>[2x]AQPTNFHDQLKFAWLAGFVDADGCINAQIVSREDYLLKYQVRVSLTVFQSTTQHFILLDIQKILGCGTVRKRNDGMSEFCVVGGTSLQTTLEKLLPYLQLKRAQAKLVL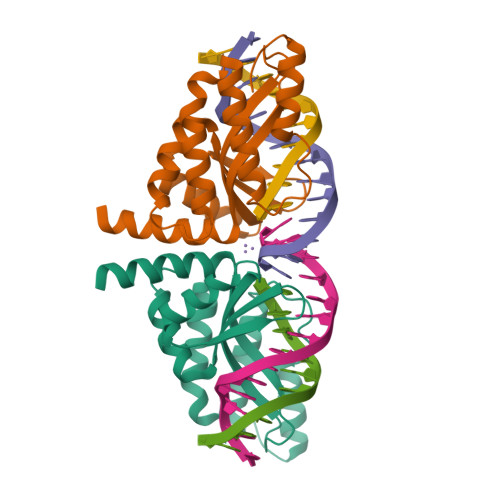QIIKKLPNTKDPSVLMEAALLADKVGLLTDGKKRTILAENVRECLKKLGHVVSAALEHHHHHH> MSFFRDLLESVVPTAYAEEPVEDVEVEQPEDAPEEEVSEETVEEEEEDDEDDDEDDEEEEETADPLDTLREECTKTAACKPFDHHFHECIERVTKEQEEPDYEHKHYKEDCIEEF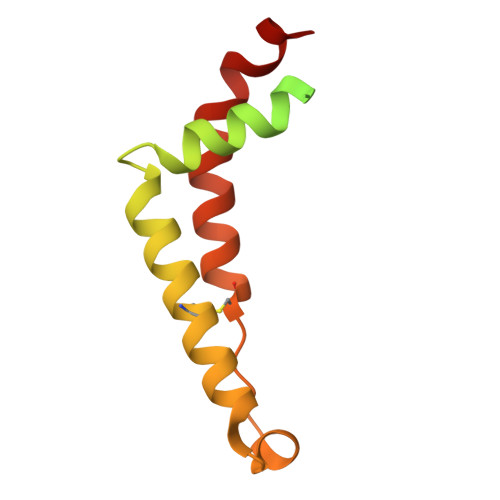FHLQHCVNDCVAPRLFNRLK>[2x]THPIIHDLENRYTSKKYDPSKKVSQEDLAVLLEALRLSASSINSQPWKFIVIESDAAKQRMHDSFANMHQFNQPHIKACSHVILFANKLSYTRDDYDVVLSKAVADKRITEEQKEAA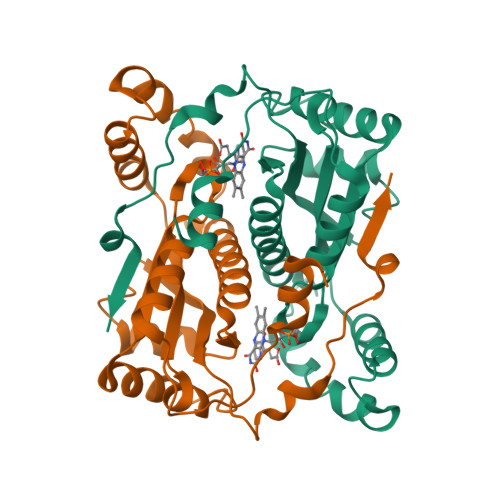FASFKFVELNCDENGEHKAWTKPQAYLALGNALHTLARLNIDSTTMEGIDPELLSEIFADELKGYECHVALAIGYHHPSEDYNASLPKSRKAFEDVITIL> AECSVDI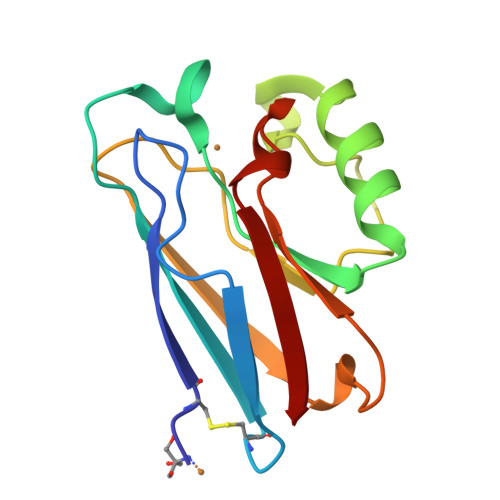QGNDQMQFNTNAITVDKSCKQFTVNLSHPGNLPKNVMGHNWVLSTAADMQGVVTDGMASGLDKDYLKPDDSRVIAHTKLIGSGEKDSVTFDVSKLKEGEQYMFFDTFPGHSALLKGTLTLK>[2x]MGSSHHHHHHSSGRENLYFQGHMHLDRQSLEKAKHLIQSGLIDTIEVGTIKGLQEIHRFLFEGLYEFAGKIRDKNI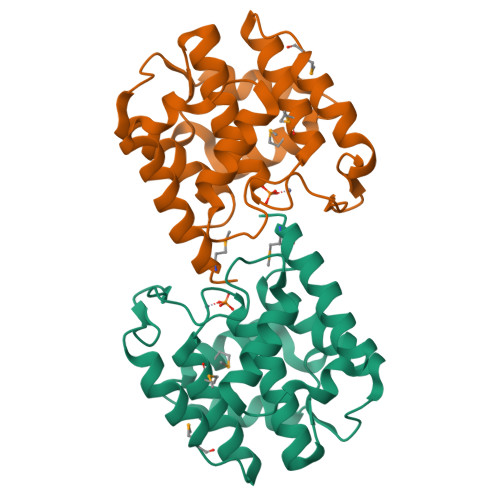AKGNFRFANCLYLDLILPRIESMPQNNFNQIVEKYVEMNIAHPFLEGNGRATRIWLDLLLKKELKKIVLWDRIDKAAYLSAMERSPVNDLEIKTLLKKHLSSNTNDPLTLIKGITQSYYYEGLGS> KKMAFTLADRVTEEMLADKAALVVEVVEENYHDAPIVGIAVVNEHGRFFLRPETALADPQFVAWLGDETKKKSMFDSKRAAVALKWKGIELCGVSFDLLLAAYLLDPAQGVDDVAAAAKMKQYEAVRPDEAVYGKGAKRAVPDEPVLAEHLVRKAAAIWELERPFLDELRRNEQDRLLVELEQPLSSILAEMEFAGVKVDTKRLEQMGKELAEQLGTVEQRIYELAGQEFNINSPKQLGVILFEKLQLPVLKKTKTGYSTSADVLEKLAPYHEIVENILHYRQLGKLQSTYIEGLLKVVRPDTKKVHTIFNQALTQTGRLSSTEPNLQNIPIRLEEGRKIRQAFVPSESDWLIFAADYSQIELRVLAHIAEDDNLMEAFRRDLDIHTKTAMDIFQV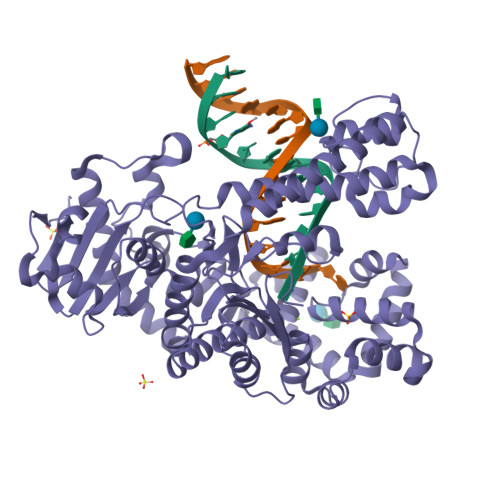SEDEVTPNMRRQAKAVNFGIVYGISDYGLAQNLNISRKEAAEFIERYFESFPGVKRYMENIVQEAKQKGYVTTLLHRRRYLPDITSRNFNVRSFAERMAMNTPIQGSAADIIKKAMIDLNARLKEERLQAHLLLQVHDELILEAPKEEMERLCRLVPEVMEQAVTLRVPLKVDYHYGSTWYDAK> RDPA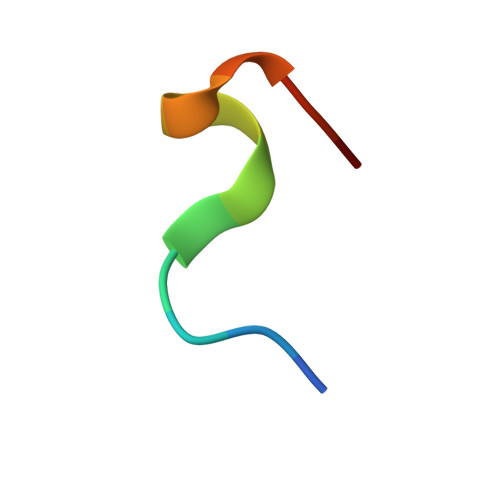PAWAHGGGX> GSHMLKGQEFAPSHQQVYAPLRADGDKPRAHLTVVRQT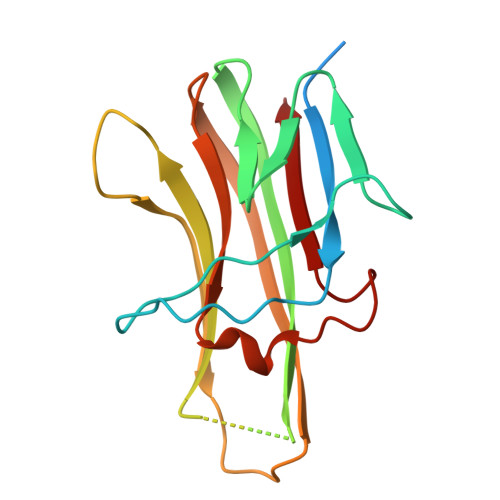PTQHFKNQFPALHWEHELGLAFTKNRMNYTNKFLLIPESGDYFIYSQVTFRGMTSECSEIRQAGRPNKPDSITVVITKVTDSYPEPTQLLMGTKSVSEVGSNWFQPIYLGAMFSLQEGDKLMVNVSDISLVDYTKEDKTFFGAFLL>GSMPKPINVRVTTMDAELEFAIQPNTTGKQLFDQVVKTVGLREVWFFGLQYVDSKGYSTWLKLNKKVTQQDVKKENPLQFKFRAKFFPEDVSEELIQEITQRLFFLQVKEAILNDEIYCPPETAVLLASYAVQAKYGDYNKEIHKPGYLANDRLLPQRVLEQHKLTKEQWEERIQNWHEEHRGMLREDSMMEYLKIAQDLEMYGVNYFEIKNKKGTELWLGVDALGLNIYEHDDKLTPKIGFPWSEIRNISFNDKKFVIKPID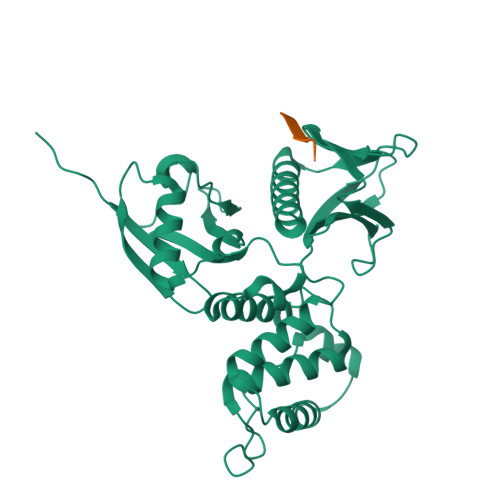KKAPDFVFYAPRLRINKRILALCMGNHELYMRRRK[4x];>[4x]NRCCDRYEEYDLE>GSVAGRIVIDDVQPVVSNGRYPAKAVVGEVVPVAATVWREGHDAVAATLVVRYHGTTYPDLADPPPGVPGADRTAVPIGDVMTPAAPVKPQRLPMSPGHTPDVFHGHFTPDRVGLWTYRVDGWGDPIASWRHNVTAKLDAGQGESELNNDLLVGARLLERAATGVPRELREALLEAAAALRAPGDPFTRAGAALSAEVSDLLAEYPLREFVTRGEQYGVWVDRPEARFSSWYEMFPRSTGGWDAEGRPVHGTFATAAEALPRIARMGFDVVYLPPIHPIGKVHRKGRNNSVTAAPGDVGSPWAIGSDEGGHDAVHPQLGTIEDFDEFVASARDLGLEVALDLALQCAPDHPWAREHPEWFTVLPDGSIAYAENPPKKYQDIYPLNFDNDPAGIYQEVLRVVRFWISHGVNIFRVDNPHTKPPNFWAWLIGQIKNENPDVLFLSEAFTRPARLYGLAKLGFTQSYTYFTWRTSKWELTEFGQEIAAKADIARPNLFVNTPDILHESLQHGGPGMFAIRAVLAATMGPAWGVYSGYELFENQPVRPGSEEYLNSEKYELRPRDFESALARGESLEPFLTRLNEIRRLHPALRELRTIRFHHVDNDALLAYSKFDPGTGDTVLVVVTLNPFGAEEATLWLDMPELGMEPYDRFWVRDEITGEEYQWGQANYVRLDPAKAVAHVLNMPLIPADKRLQLLRRE[2x]

GlgE is a maltosyl transferase that transfers maltose from a maltose-1-phosphate (maltose-1P) donor to α-(1–4) glucan chains. GlgE is essential for M. tuberculosis and its depletion leads to pleiotropic stress effects and eventually cell death. GlgE is proposed to catalyse the transfer of maltosyl units to α-glucan chains through a double-displacement reaction in which an aspartate residue acts as a nucleophile forming an β-maltosyl-enzyme intermediate, while a glutamate residue is thought to protonate the phosphate and deprotonate the acceptor, acting like an acid/base catalytic residue16. Each of the protomers of M. thermoresistibile GlgE contains 5 domains and 2 inserts that have been described extensively in the first reported GlgE structure and therefore we will focus on the particular characteristics of M. thermoresistibile GlgE.

In an attempt to obtain a maltosyl-GlgE intermediate state, GlgE was co-crystalized with maltose-1P. We could not observe the maltosyl-GlgE intermediate but instead we found maltose bound to only one of the active sites of the dimer. The fact that maltose was present instead of maltose-1P is most likely due to GlgE slowly degrading maltose-1P to maltose, since maltose-1P was free of maltose contamination and we confirmed its stability at different temperatures for long periods of time. Significant conformational changes were however visible in the structure especially in the S domain of the protomer with bound maltose. The S domain of this protomer exhibits conformational changes with several residues of α1 (V132–L136) and α2 (S146–150) losing their helical conformation. Moreover, all four helices comprising the S domain of the maltose-bound protomer were found to be shifted with a maximum distance of ~6.5 Å when compared to both the maltose co-crystallization and the apo structure. This brings domain S of the maltose containing protomer closer to loop 2 of domain B of the “apo” protomer. Unfortunately, the majority of domain B, including loop 2 and the antiparallel β-strand lid, is not seen clearly in the maltose-1P co-crystallization structure “apo-protomer” and thus it could not be modeled.>EVIERARRLLRELADLAEERGDEGVAAAAREVERLVAERGDRELAAVVAALAAAALLALERGDEVLARLAAAAAVLVAKRERGKVAKAVAELARLARLALERGDEETARLVAEVALLVASKGDDELAEKVAELAREARDALEAG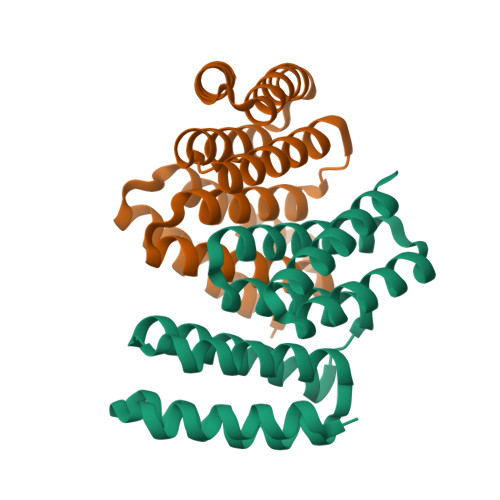DRERAREAAEEALRVAREAE[4x]>GSMSELSVATGAVSTASSSIPMPAGVNPADLAAELAAVVTESVDEDYLLYECDGQWVLAAGVQAMVELDSDELRVIRDGVTRRQQWSGRPGAALGEAVDRLLLETDQAFGWVAFEFGVHRYGLQQRLAPHTPLARVFSPRTRIMVSEKEIRLFDAGIRHREAIDRLLATGVREVPQSRSVDVSDDPSGFRRRVAVAVDEIAAGRYHKVILSRCVEVPFAIDFPLTYRLGRRHNTPVRSFLLQLGGIRALGYSPELVTAVRADGVVITEPLAGTRALGRGPAIDRLARDDLESNSKEIVEHAISVRSSLEEITDIAEPGSAAVIDFMTVRERGSVQHLGSTIRARLDPSSDRMAALEALFPAVTASGIPKAAGVEAIFRLDECPRGLYSGA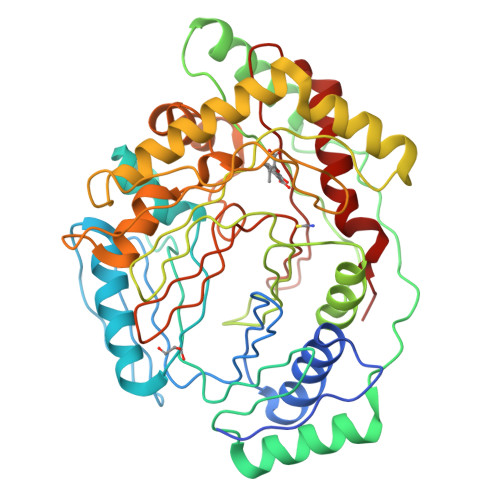VVMLSADGGLDAALTLRAAYQVGGRTWLRAGAGIIEESEPEREFEETCEKLSTLTPYLVAR[4x]D-fructose | C6 H12 O6 | 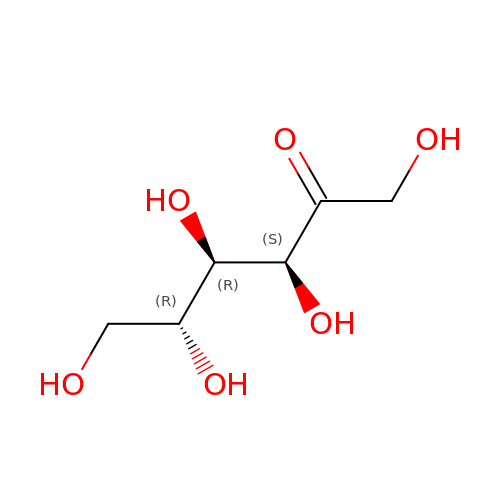BJHIKXHVCXFQLS-UYFOZJQFSA-N> MSNAFEYLRTYVESTTETDAAVARAREDAAEFGLPAPDEMTGQLLTTLAATTNGNGSTGAIAITPAAGLVGLYILNGLADNTTLTCIDPESEHQRQAKALFREAGYSPSRVRFLLSRPLDVMSRLANDSYQLVFGQVSPMDLKALVDAAWPLLRRGGALVLADALLDGTIADQTRKDRDTQAARDADEYIRSIEGAHVARLPLGAGLTV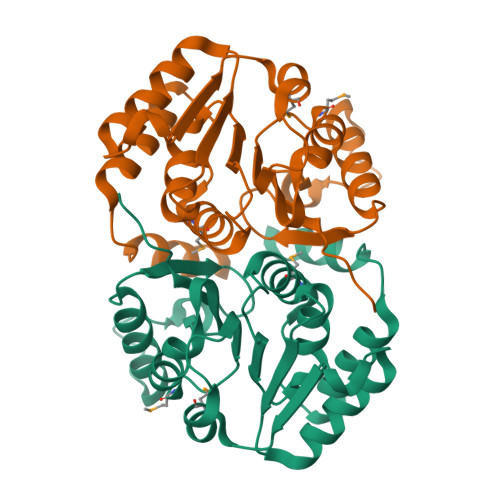VTKALEHHHHHH> WGALGHATVAYVAQHYVSPEAASWAQGILGSSSSSYLASIASWADEYRLTSAGKWSASLHFIDAEDNPPTNCNVDYERDCGSSGCSISAIANYTQRVSDSSLSSENHAEALRFLVHFIGDMTQPLHDEAYAVGGNKINVTFDGYHDNLHSDWDTYMPQKLIGGHALSDAESWAKTLVQ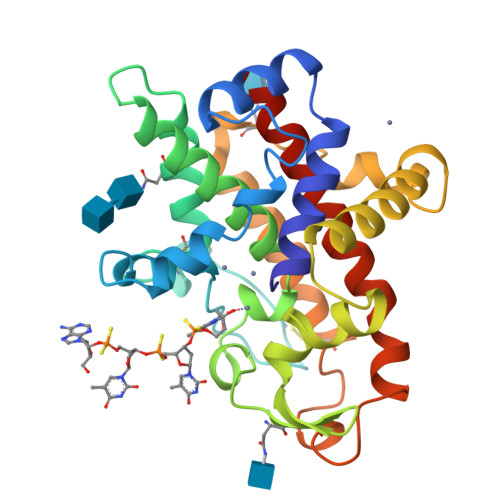NIESGNYTAQAIGWIKGDNISEPITTATRWASDANALVCTVVMPHGAAALQTGDLYPTYYDSVIDTIELQIAKGGYRLANWINEIHGSEIAK>XETAAFAALRKPVDVAFGRNYVPTWAFDHIKYFNGGNEIQLHLDKYTGTGFQSKGSYLFGHFSMQMKLVPGDSAGTVTAFYLSSQNSEHDEIDFEFLGNRTGQPYILQTNVFTGGKGDREQRIYLWFDPTKEFHYYSVLWNMYMIVFLVDDVPIRVFKNCKDLGVKFPFNQPMKIYSSLWNAD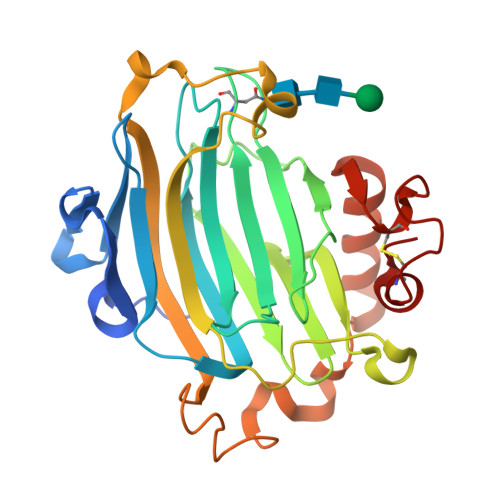DWATRGGLEKTDWSKAPFIASYRSFHIDGCEASVEAKFCATQGARWWDQKEFQDLDAFQYRRLSWVRQKYTIYNYCTDRSRYPSMPPECKRDRDI[2x]> MAAALSEQLAELEKRSGGRLGVAVLDTATGRRFGYRGDERFPMCSTFKALLAAAVLARVDQGKENLDRRITYGKEDLVDYSPVTEKHVGDGMTVAELCEAAITYSDNTAANLLLEALGGPAALTAFLRSIGDNVTRLDRWEPELNTAAPGDPRDTTTPAAMAATLRTLLLGDVLSPASRQQLVDWLIANKTGDKRLRAG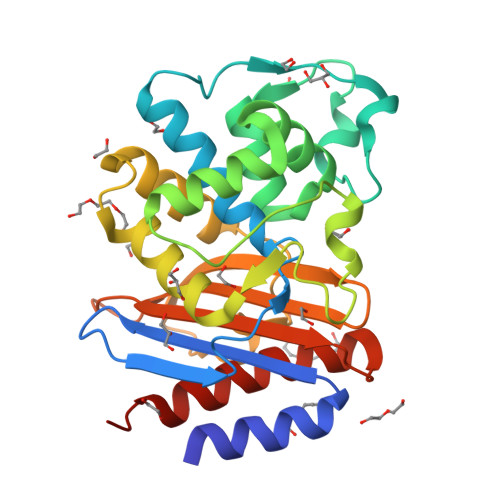LPADDRVGDKTGTGEHGTTNDIAVIWPPNRAPILVAVYLTESQVDADARDAVIAEVARLVVAAWHHHHHH Fungal immunomodulatory proteins (FIPs) are a group of low-molecular-weight (MW) proteins investigated as potential anti-tumor drugs. FIP-nha (from Nectria haematococca) contains two glycosylation sites at positions N5 and N39. In this study, the impact of glycosylation on the bioactivity and biochemical characteristics of FIP-nha (from Nectria haematococca) is described. Taken together, these findings indicate that glycosylation of FIP-nha impacts its thermostability and digestion resistance.

To study the impact of glycosylation on functionality of rFIP-nha, two single mutants (N5A and N39A) and one double mutant (N5+39A) were constructed to remove glycosylation sites. The SDS-PAGE results showed that the purified WT, N5A and N39A were partially glycosylated, while the N5+39A variant was indeed unglycosylated. However, we only managed to obtain crystals and solved the structures of WT, N39A and N5+39A. Unfortunately, none of the structures contained a density indicative of N-glycosylation. SLS and native-PAGE results suggested that rFIP-nha and its variants were all homogeneously tetrameric in the solution. The Tm values for WT, N5A, N39A and N5+39A were 82.2 °C, 81.4 °C, 80.7 °C and 80.1 °C, respectively. Highly glycosylated forms of rFIP-nha seemed more stable, indicating that N-glycosylation might contribute to thermostability. The stability of rFIP-nha during pepsin digestion was in this order: WT (T1/2 11.6 min) > N39A (T1/2 1.9 min) > N5A (T1/2 1.3 min) > N5+39A (T1/2 0.5 min). Double glycosylation significantly enhanced the pepsin resistance. Resistance to trypsin digestion is shown in Figure 6: N5A (T1/2 longer than 240 min) > WT (T1/2 89.3 min) > N5+39A (T1/2 13.9 min) > N39A (T1/2 8.1 min). However, there were no significant differences in tumor mitochondrial metabolism inhibition among the rFIP-nha variants toward the tested tumor cell lines.

>[4x]GPLGSMATTADSAVLFYIVASQKKLSFDYTPNWGRGSPNSYIDALTFPRVLTNKPYKYRVVKAGQDLGVRDSYSVQSDGSQKVNFLEYNAGRGIADTQTIQVYVVDPDNGNQYLVAQWKHHHHHH2-{2-deoxy-5-O-[(R)-hydroxy{[(R)-hydroxy(phosphonooxy)phosphoryl]oxy}phosphoryl]-beta-D-erythro-pentofuranosyl}-6-methylisoquinoline-1(2H)-thione 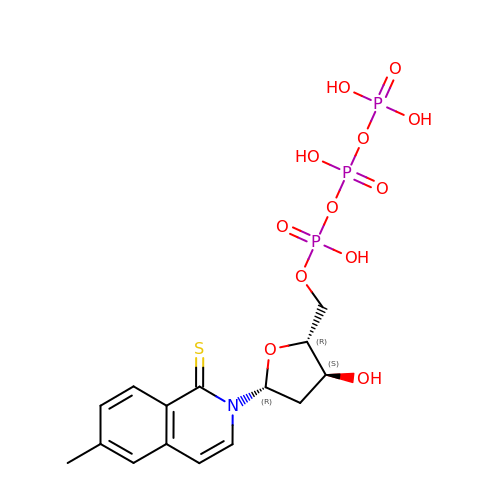| C15 H20 N O12 P3 S | HHAKTXADNAZKDV-BFHYXJOUSA-N>[6x]MGGEVEEPEPQMVLSPLTSAAIFLVVTIDSGGEDTVRDLLSDVASLERAVGFRAQPDGRLSCVTGIGSEAWDRLFSGARPAGLHPFRELDGPVHRAVATPGDLLFHIRASRLDLCFALATEIMGRLRGAVTPQDEVHGFKYFDERDMLGFVAGTENPTGAAA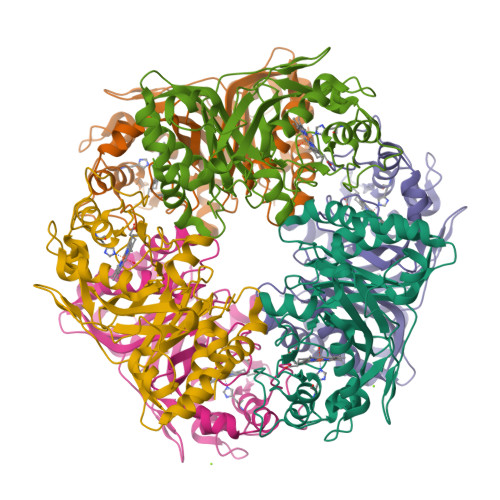RRAVLVGAEDPAFAGGSYAVVQKYLHDIDAWEGLSVEAQERVIGRRKMTDVELSDDVKPADSHVALTSVTGPDGSDLEILRDNMPFGSVGREEFGTYFIGYARTPEVTETMLERMFLGTASAPHDRILDFSTAVTGSLFFTPAADFLEDLSARP> MEQNLFALSLDDTSSVRGSLLDTKFAQTRVLLSKAMAGGDVLLDEYLYDVVNGQDFRATVAFLRTHVITGKIKVTATTNISDNSGCCLMLAINSGVRGKYSTDVYTICSQDSMTWNPGCKKNFSFTFNPNPCGDSWSAEMISRSRVRMTVICVSGWTLSPTTDVIAKLDWSIVNEKCEPTIYHLADCQNWLPLNRWMGKLTFPQGVTSEVRRMPLSIGGGAG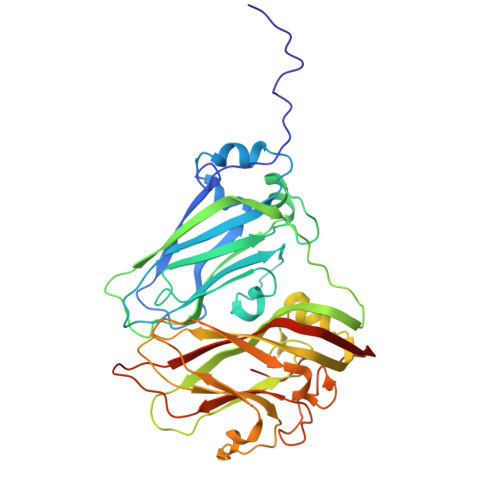ATQAFLANMPNSWISMWRYFRGELHFEVTKMSSPYIKATVTFLIAFGNLSDAFGFYESFPHRIVQFAEVEEKCTLVFSQQEFVTAWSTQVNPRTTLEADGCPYLYAIIHDSTTGTISGDFNLGVKLVGIKDFCGIGSNPGIDGSRLLGAIAQ>[2x]MHHHHHHMAKIIFPEDFIWGAATSSYQIEGAFNEDGKGESIWDRFSHTPGKIENGDTGDIACDHYHLYREDIELMKEIGIRSYRFSTSWPRILPEGKGRVNQKGLDFYKRLVDNLLKANIRPMITLYHWDLPQALQDKGGWTNRDTAKYFAEYARLMFEEFNGLVDLWVTHNEPWVVAFEGHAFGNHAPGTKDFKTALQVAHHLLLSHGMAVDIFREEDLPGEI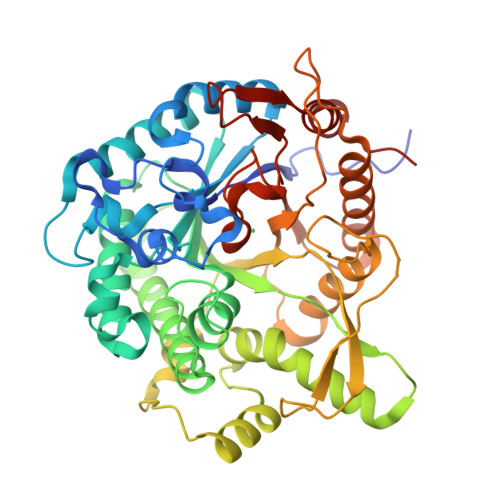GITLNLTPAYPAGDSEKDVKAASLLDDYINAWFLSPVFKGSYPEELHHIYEQNLGAFTTQPGDMDIISRDIDFLGINYYSRMVVRHKPGDNLFNAEVVKMEDRPSTEMGWEIYPQGLYDILVRVNKEYTDKPLYITENGAAFDDKLTEEGKIHDEKRINYLGDHFKQAYKALKDGVPLRGYYVWSLMDNFEWAYGYSKRFGLIYVDYENGNRRFLKDSALWYREVIEKGQVEAN> MSRSAFSSRGALLFSSAPLQCQRRWVTRLYTSYYTGVLYPNQLVQPKQRLPADVSVSAILQKRSEPEAAAERGSNKGDKVDVSKGEKTPRVSWDDADSTDVMRVDNTQQLKEAPQVERPYVPLGEVAKLELQGDYYMEGGMFQEALEHYGVVAKAYNYAYPENHAQRIGIRIKLSAAFRQTGRLESSLANIEEVLRMLDASTRPSLELICEALLELGITREALGMKREATEAYEEALEVVNSFHNWGESHRMLRLLPRLGRRFNYNFEEKFVYFSPFDYDRTFALVDQCLERAETIFNEIGDVEGAIRVLQQRKEMIDKKFFNMRDFAGRIHTMRGHWKRRAQHLTNAPTPDELLRYSPTIHQVHRDFKYELTAPIGREKEVMPGVNRLVLDMGNPYRRRGR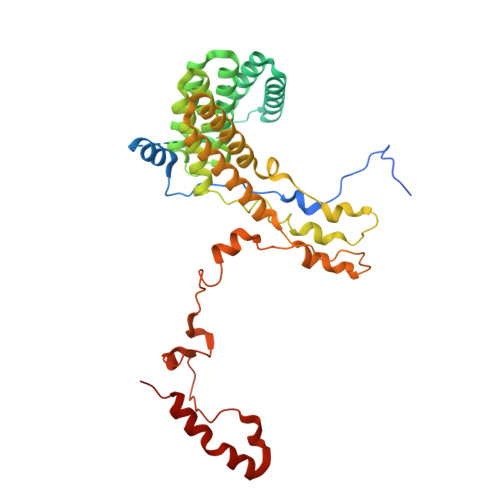LSNKMLKDADHKFANYVRQKEYNE> MTQVRETVSFKAGDVILYPGVPGPRDRAYRVLEGLVRLEAVDEEGNALTLRLVRPGGFFGEEALFGQERIYFAEAATDVRLEPLPENPDPELL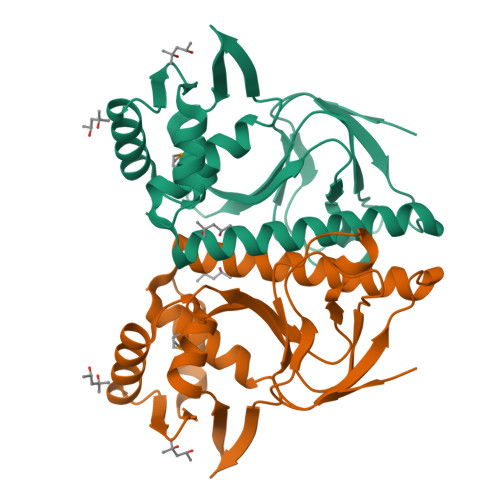KDLAQHLSQGLAEAYRRIERLATQRLKNRMAAALLELSETPLAHEEEGKVVLKATHDELAAAVGSVRETVTKVIGELAREGYIRSGYGKIQLLDLKGLKELAESRGQGR ethyl 4-oxidanylidene-4-[4-(trifluoromethyl)-2,3-dihydroindol-1-yl]butanoate | C15 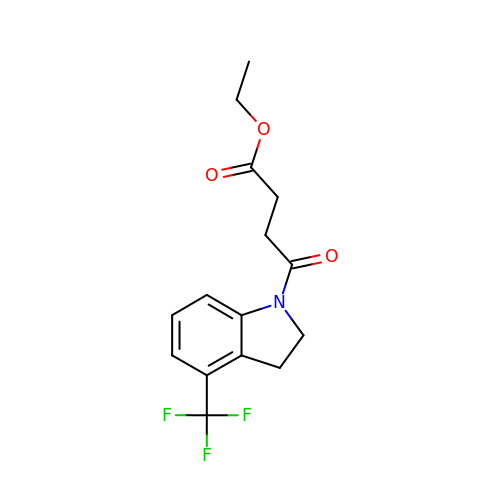H16 F3 N O3 | ZUBJCDWADSBMLA-UHFFFAOYSA-N> MGVPKFFRYISERYPCLSELAREHCIPEFDNLYLDMNGIVHNCSHPDDNNIHFHLE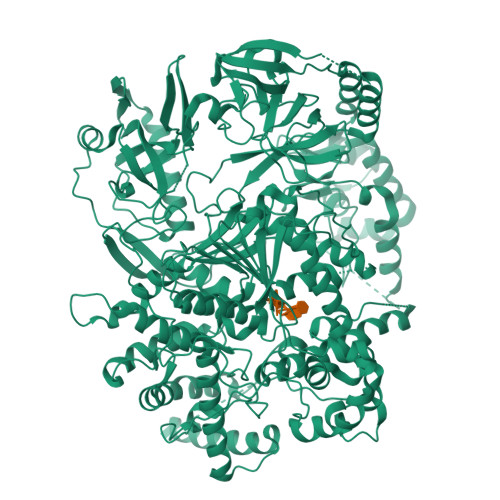EEQIFQEIFNYVDKLFYLIKPQRLFFLSVDGVAPRAKMNQQRSRRFRTAREAEQQEAKAAQRGELREHERFDSNCITPGTEFMVRLQEGLRAFLKTKISTDPLWQRCTVILSGQEAPGEGEHKIMDYIRYMKTQPDYDPNTRHCLYGLDAALIILGLCTHELHFVVLREEVKFGRNVKRTSVEETRFFLLHLGLLREYLELEFDALRTDEHKLDIAQLIDDWVLMGFLVGNDFIPHLPCLHISSNALPLLYRTYIGIYPTLGGNINENGKLNLRRLQIFISALTEVELDHFKEHADDLKYMNNKSEAFDMDVGEITESQNLDSDLGALINKSMLLYDDDSEEDCSDENAVLLKEFQNYKRNFYRNKFKRDPNDELIEELCHHYVNALQWVLDYYYRGVQSWDWYYPFHYTPFISDLKNIEQVEIAFHMGTPFLPFQQLLAVLPAASAKLLPVAYHDLMLLPTSPLAEFYPLEFESDLNGKKHDWEAVVLIPFIDEGRLLAAMLPCEAQLSLEERERNRHGPMYVYKYSTVAQGPMPAYPPLRALPVLYCTEVAKWSHEIAVNLPYSVCIELPNAARTVFFPGFPTMQHLPFDFELRNDRVKVFEQVSRNQNIVLKPRKRQLEDTLTAVASQYLGKVIHVGWPHLVKAIVVRVATRDQRVDSEGITLNDSRRFDSECKALQEHFINRMGIQFANYDVLVYVRTFAGNSTEFRDKGALMVRDSWSSSVTGYPAQGVVADLTVWERMRKNFLNVEHYFPVGSTIFLITDPYYGSEGTVQDPRLAYTNGRIQVSIMVRPEPKVNAARQLQEERDRDYLSTFQVCNLLRISGRTLGRLSGTVWVVLGPRRQKMENVTKHNIGLQLKYPRQNEERAGYCFRTNNQWYYSSLAVDLMRNYCQRYPDVIDFFGDSNDRAEFVFEQDVFPNAVGHRRVEELANWVRQQPHMKVERISCGSKTVCRETIELLIAAVDDLRSLPVKHVKLQVKPHLLIKPNVTLPDVYRSKRPVRLFDRVVIVRTIYMVPVGTKGTVIGIHPVTDPNPVRLECVHAVDTFCKVLFDSPVPNCNNIHGIAEDRVYKVPEIALVIIK> HHHHHHMTFPGDTAVLVLAAGPGTRMRSDTPKVLHTLAGRSMLSHVLHAIAKLAPQRLIVVLGHDHQRIAPLVGELADTLGRTIDVALQDRPLGTGHAVLCGLSALPDDYAGNVVVTSGDTPLLDADTLADLIATHRAVSAAVTVLTTTLDDPFGYGRILRTQDHEVMAIVEQTDATPSQREIREVNAGVYAFDIAALRSALSRLSSNNAQQELYLTDVIAILRSDGQTVHASHVDDSALVAGVNNRVQLAELASELNRRVVAAHQLAGVTVVDPATTWIDVDVTIGRDTVIHPGTQLLGRTQIGGRCVVGPDTTLTDVAVGDGASVVRTHGSSSSIGDGAAVGPFTYLRPGTALGADGKLGAFVEVKNSTIGTGTKVPHLTYVGDADIGEYSNIGASSVFVNYDGTSKRRTTVGSHVRTGSDTMFVAPVTI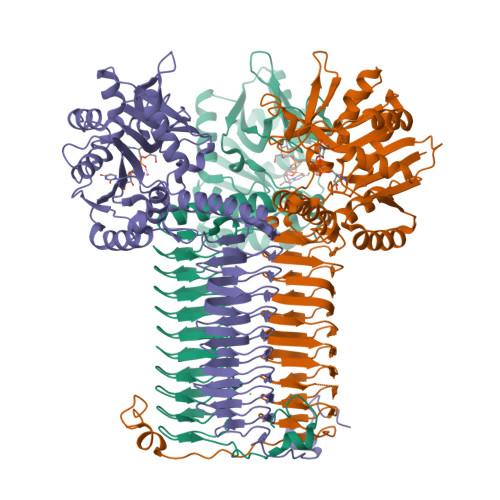GDGAYTGAGTVVREDVPPGALAVSAGPQRNIENWVQRKRPGSPAAQASKRASEMACQQPTQPPDADQTP>MAIKVIEEKCIGCSKCQKSCPFDAITIENKIAVIGDACTNCGTCIDVCPTEAILQEGTEKIVRDLSMYKGVWVFAEQREGKIMPVVFELLGEGKKLANE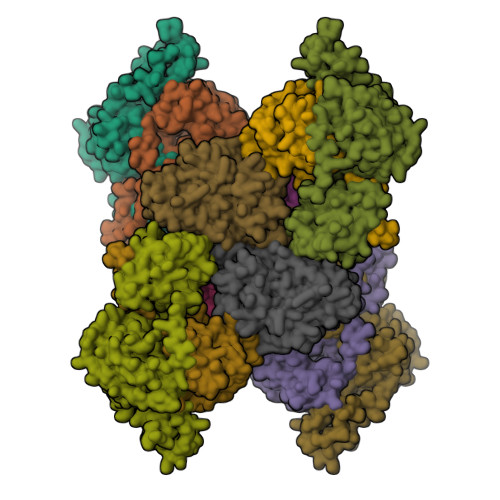IGTELCAILCGSNVAELTDELFAYGADKVYLADAPELEKYTTDGYSKIINEAIGLYKPEIVLYGATHIGRDLAPCLAVKVNTGLTADCTKLEIDPDDKKIRQTRPAFGGNLMATIVCPGSRPQMSTVRPGVMDKAAYDPSQKGEVIKLDATFNEGDIRTKVLEIVKTTTDNISISDADFIVSGGMGLGKPEGFELLKQLADKLGGTVATSRACVDAGWADHAQQVGQTGTTVKPQIYFACGISGAIQHIAGMQDSDIIIAINKNENAPIFEVADYGIVGDLYKVIPAIIEELDKIGK[2x];>MRILVCAKQVPDTNEVKIDPKTGTMIREGVPSILNPDDANALEAALVIKDENPGTEVIVMTMGPPQASEMLRECLAMGADEAYLLSDRAFGGADTWATSATLAAGIKKVKKVDLVLAGRQAIDGDTAQVGSQIAQRLKMPVVTYVEDIKIEDKKAIVHRQMEDGYEVIEVQLPCLLTCVKELNDPRYMSVGGIMDAYEQPITIWNHEDIGLSPEACGLNASPTQVFRSFSPPAKGGGEMITGTTVNEVAGSLVSKLKEKHII[2x];>MYFSEQNKMIRKLARDFAEKELTTEILDEVEESGEFPQEILDKMAKFGFFGIKIPKSLGGSGGDHMSYVICMEEFARVSGVASVYLSSPNSLAGGPLLLSGTEEQIEKYLKPIITGKKKLAFALTEPGAGSDAGGMSTTAVDMGDYYLLNGRKTFITMAPLCDDAVIYAKTDMSKGTRGISAFIVDLKSEGVSMGKNEHKMGLIGCATSDIIMEDVKVPKENRLGEVNKGFSNAMKTLDVGRLGVASQSIGVAQGALDEAIKYAKERKQFGKRIADFQAIAFMIADMATKLEAAKLLVYNAASLMDNKKNATKEASMAKFYASEICNEICAKAVQIHGGYGYIKEYKVERMYRDCRVFTIYEGTSQVQQMVISGMLLKK[2x]>GPMPGKKFVARVVEARAEDVGKRVVIIPKGIKVGDVVEVKKV[2x]

Here, we study fold transition between distinct β-barrels by protein engineering and structural biology technique. Here, we discover that the previously reconstructed ancient DPBB sequence could also adopt a β-barrel fold named Double-Zeta β-barrel (DZBB), as a metamorphic protein. The DZBB fold is not found in any modern protein, although its structure shares similarities with RIFT and OB. Furthermore, the reconstructed OB fold could also be converted to the four-stranded SH3 fold by a simple circular permutation. Thus, these ancient β-barrel folds (DPBB, RIFT, OB, and SH3) could be readily interconverted by a few feasible mutations through the missing-link fold, DZBB, indicating their significantly close evolutionary relationships.

To test this assumption, we conducted the reverse engineering by replacing segment 1 of design-13 and design-16 with the 8-amino acid sequence forming the Z-loop of design-2 (the 3rd generation mutants: design-18 (tkoL2_v1.2_Z) and design-19 (mkaL2_v1.2_Z)). SEC and CD experiments demonstrated that both mutants folded and had moderate thermal stabilities. The crystal structures of design-18 and design-19 revealed that they adopt the DZBB fold even without the α1 region (segment 2). These results demonstrated that the segment 1 is sufficient to archive the fold-change from DZBB to OB. Most DNA molecules did not migrate from the well when mixed with the proteins with the stable DZBB fold (design-2, -18, and -19) and RIFT fold (design-3 and -4), indicating that these proteins formed large aggregates with dsDNA. In particular, design-2, -18, -19, -3, and -4 interacted with dsDNA even in high salt conditions (500 mM NaCl). Design-2, -18, -19, -3, and -4 might interact with the phosphate groups in the DNA backbone in a similar way to the sulfate ions in the crystal structures of DZBB.>TGSKPFTVPILTVEEMTNSRFPIPLEKLFTGPSGAFVVQPQNGRCTTDGVLLGTTQLSPVNICT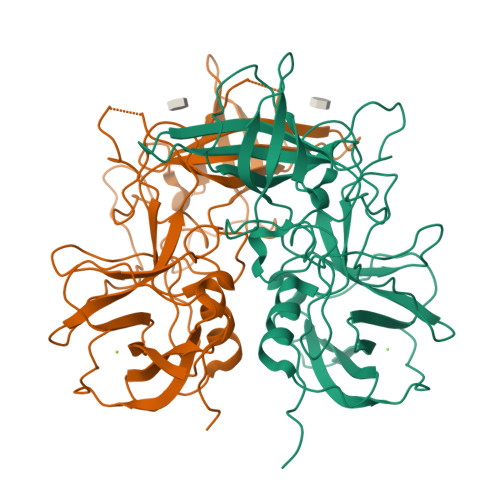FRGDVTHIAGSRNYTMNLASLNWNNYDPTEEIPAPLGTPDFVGKIQGLLTQTTKGDGSTRGHKATVYTGSAPFTPKLGSVQFSTDTEDDFETHQNTKFTPVGVIQDGSTTHRNEPQQWVLPSYSGRNVHNVHLAPAVAPTFPGEQLLFFRSTMPGCSGYPNMDLDCLLPQEWVQHFYQEAAPAQSDVALLRFVNPDTGRVLFECKLHKSGYVTVAHTGQHDLVIPPNGYFRFDSWVNQFYTLAPM[2x]> GPLGSMLKLSELHDVFQRHPELELKYLNMMKMAITGKESICLPFNFHSHR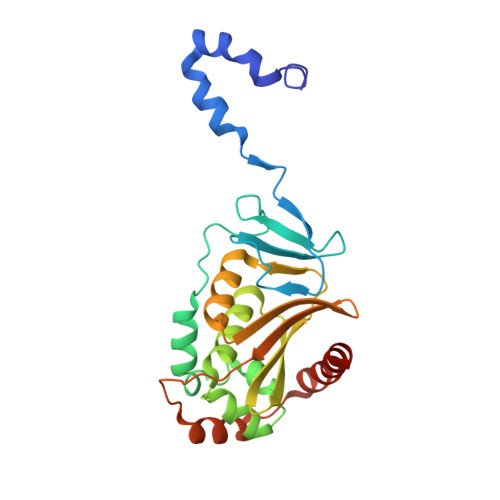QHTCLDISPYGNEQVSRIACTSCEDNRILPTASDAMVAFINQTSNIMKNRNFYYGFCKSSELLKLSTNQPPIFQIYYLLHAANHDIVPFMHAEDGRLHMHVIFENPDVHIPCDCITQMLTAAREDYSVTLNIVRDHVVISVLCHAVSASSVKIDVTILQRKIDEMDIPNDVSESFERYKELIQELCQ>AHKKIFLVEDNKADIRLIQEALANSTVPHEVVTVRDGMEAMAYLRQEGEYANASRPDLILLDLNLPKKDGREVLAEIKSDPTL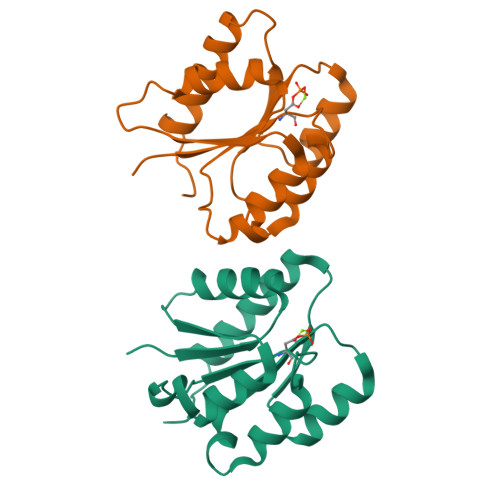KRIPVVVLSTSINEDDIFHSYDLHVNCYITKSANLSQLFQIVKGIEEFWLSTATLPS[2x]> FACKTANGTAIPIGGGSANVYVNLAPVVNVGQNLVVDLSTQIFCHNDYPETITDYVTLQRGSAYGGVLSNFSGTVKYSGSSYPFPTTSETPRVVYNSRTDKPWPVALYLTPVSSAGGV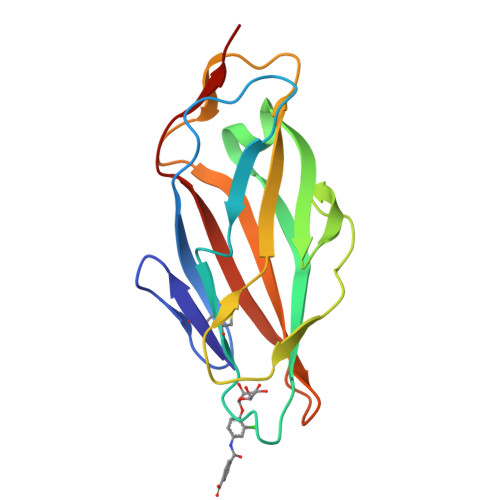AIKAGSLIAVLILRQTNNYNSDDFQFVWNIYANNDVVVPTGL METHYL 4-{[({[(2R,5S)-5-{[(2S)-2-(AMINOMETHYL)PYRROLIDIN-1-YL]CARBONYL}PYRROLIDIN-2-YL]METHYL}AMINO)CARBONYL]AMINO}BENZOATE 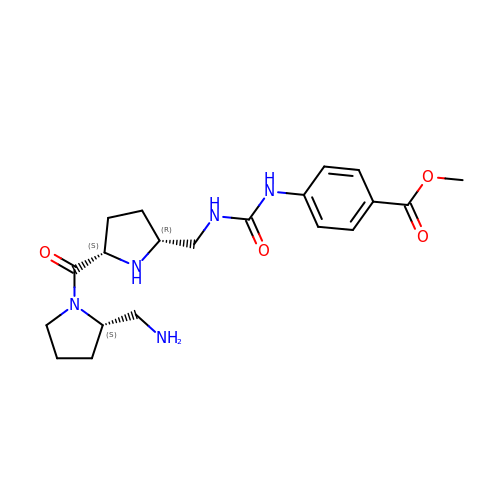| C20 H29 N5 O4 | USDCNOQKDUFKRD-IKGGRYGDSA-N>[4x]GPGSMAKPAKRVAVTGAAGQIAYSLLFRIANGDLLGKDQPVILQLLDLPQAQAAVKGVVMELDDCAFPLLAGVVITDDPKVAFKDADVALLVGARPRSKGMERKDL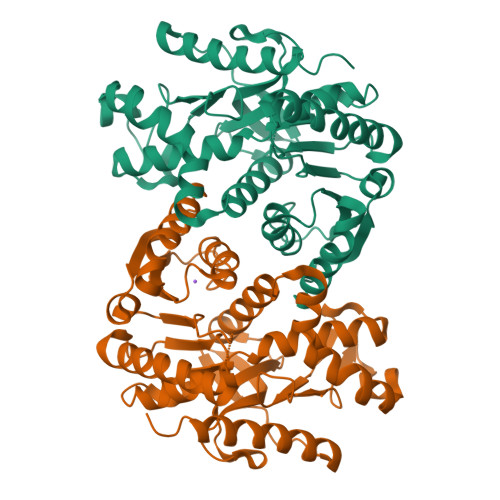LSANAEIFTVQGAALNEVASRDVKVLVVGNPANTNAYIAMKSAPDLPKKNFTAMLRLDHNRALSQLAAKSGKPVASIEKLAVWGNHSPTMYPDFRFATAEGESLLKLINDDVWNRDTFIPTVGKRGAAIIEARGLSSAASAANAAIDHVRDWVLGTNGKWVTMGIPSDGSYGIPEDIIYGVPVICENGEYKRVEGLEIDAFSREKMDGTLAELLEERDGVAHLLK> HHHHHHMEEEAETEEQQRFSYQQRLKAAVHYTVGCLCEEV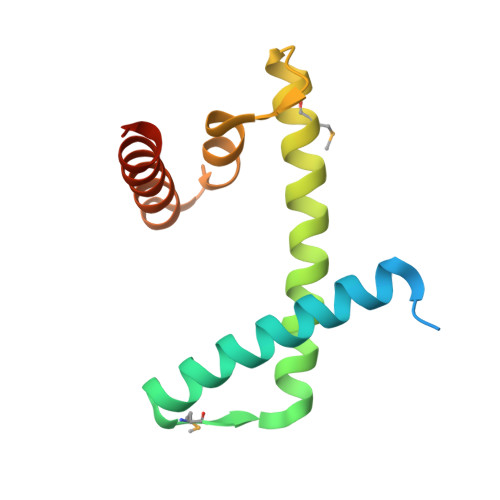ALDKEMQFSKQTIAAISELTFRQCENFAKDLEMFARHAKRTTINTEDVKLLARRSNSLLKYITDKSEEIAQINLERKAQK>MSLEDCRISRVELYALADENAPPIPWADNQEPLLYTNNIVRLFTEDGTEGLGATMSYTENFFDRCIIESLRTIVPGLIGKNPLMTQELNNWLGARCTWGGLPAKSPIDIAAWDIKGKKAGMPLYMLLGGARTKIKSYASTPMFDTVEEYFPYIDDCIEHGFTAIKLHCYCVYDKDVALVEAVEAKYGTSGIRFMLDTAGFYTPEQAMKMAKWMERHNWEWLEAPVSDYDFKTYQRLVANTDLEISSHGNCLLTLQEVTHALSTGMWSDVRQDATVCGGITQLNKCF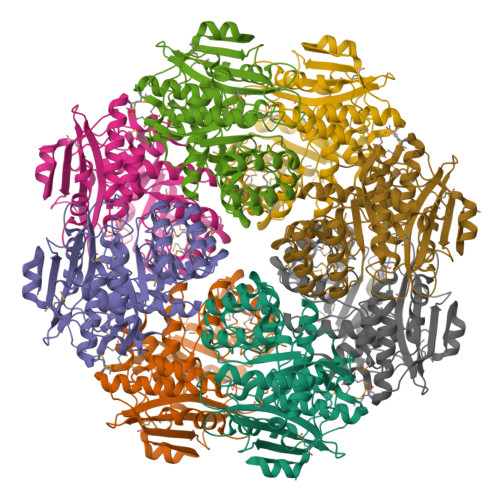AIAAGHSKNLEIQSMGYTLTQAANLHVALAHDNCNFFEQFYPYEAFELASKTQIRTDKEGYVHAPAGNGLGVEMDWDAVKEASFASYVFEEGHHHHHH[8x]>SNAQIDGFVRTLRARPEAGGKVPVF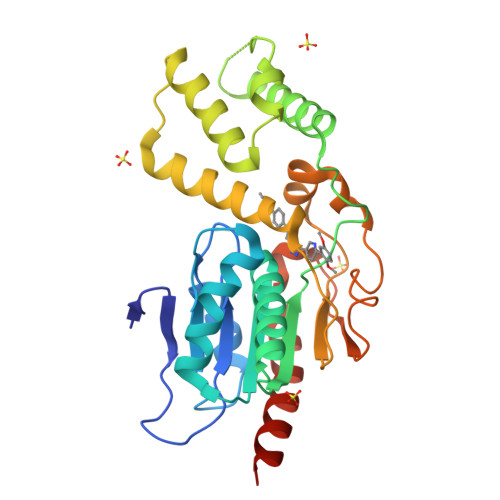VFHPAGGSTVVYEPLLGRLPADTPMYGFERVEGSIEERAQQYVPKLIEMQGDGPYVLVGWSLGGVLAYACAIGLRRLGKDVRFVGLIDAVRAGEEIPQTKEEIRKRWDRYAAFAEKTFNVTIPAIPYEQLEELDDEGQVRFVLDAVSQSGVQIPAGIIEHQRTSYLDNRAIDTAQIQPYDGHVTLYMADRYHDDAIMFEPRYAVRQPDGGWGEYVSDLEVVPIGGEHIQAIDEPIIAKVGEHMSRALGQIEADRTSEVGKQ[2x]9-oxo-N-[[(2R,3R,4R,5R,6S)-3,4,5-trihydroxy-6-methyl-piperidin-2-yl]methyl]fluorene-1-carboxamide 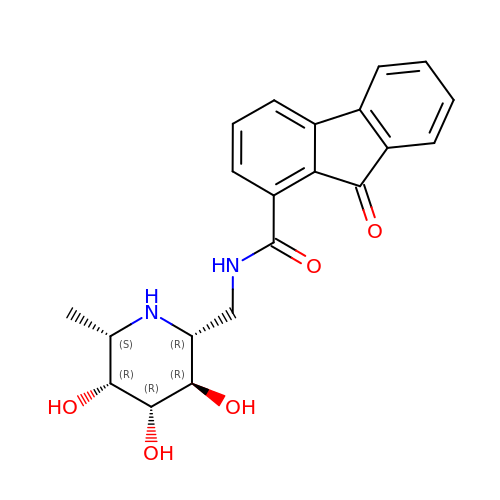| C21 H22 N2 O5 | NQPIYVRYYGVNCF-KOOFZGQNSA-N>[2x]GHMVTMSTEPVSASDKYQKISQLEHILKRPDTYIGSVETQEQLQWIYDEETDCMIEKNVTIVPGLF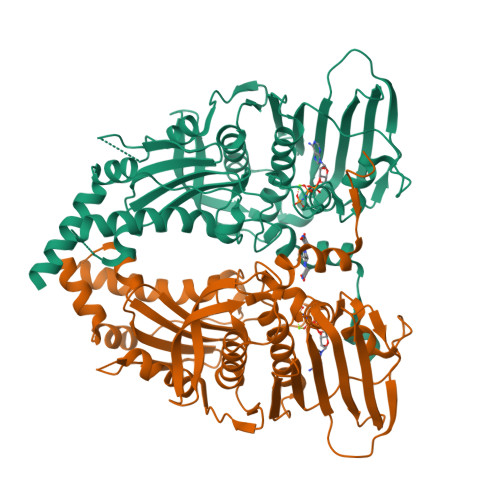KIFDEILVNAADNKVRDPSMKRIDVNIHAEEHTIEVKNDGKGIPIEIHNKENIYIPEMIFGHLLTSSNYDDDEKKVTGGRNGYGAKLCNIFSTEFILETADLNVGQKYVQKWENNMSICHPPKITSYKKGPSYTKVTFKPDLTRFGMKELDNDILGVMRRRVYDINGSVRDINVYLNGKSLKIRNFKNYVELYLKSLEKKRQLDNGEDGAAKSDIPTILYERINNRWEVAFAVSDISFQQISFVNSIATTMGGTHVNYITDQIVKKISEILKKKKKKSVKSFQIKNNMFIFINCLIENPAFTSQTKEQLTTRVKDFGSRCEIPLEYINKIMKTDLATRMFEIADANEENALK> GPLGSDLKDAEAVQKFFLEEIQLGEELLAQGDYEKGVDH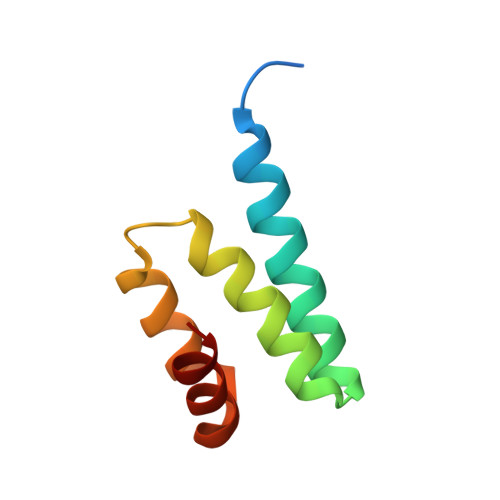LTNAIAVCGQPQQLLQVLQQTLPPPVFQMLLTKL>[2x]GSHMKKVIIAGNGPSLKEIDYSRLPNDFDVFRCNQFYFEDKYYLGKKCKAVFYNPSLFFEQYYTLKHLIQNQEYETELIMCSNYNQAHLENENFVKTFYDYFPDAHLGYDFF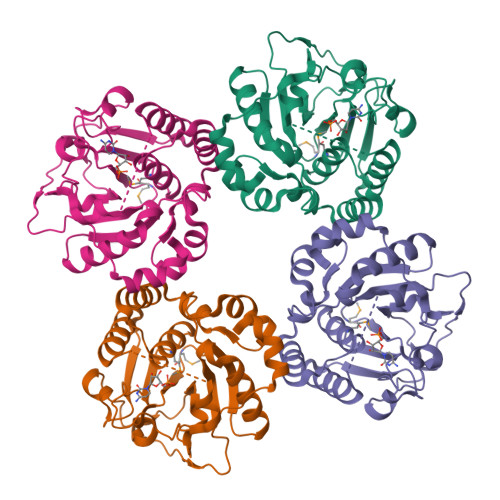KQLKDFNAYFKFHEIYFNQRITSGVYMCAVAIALGYKEIYLSGIDFYQNGSSYAFDTKQKNLLKLAPNFKNDNSHYIGHSKNTDIKALEFLEKTYKIKLYCLCPNSLLANFIGLAPNLNSNFIIQEKNNYTKDILIPSSEAYGKFSKNIN> GSRTAELQAEIDDTVGIMR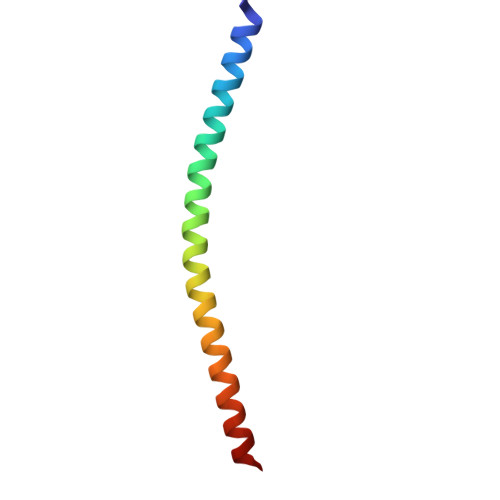DNINKVAERGERLTSIEDKADNLAVSAQGFKRGANRVRKAMW>[2x]MQTRSSRMAGFGHAVPARCVDNAEIEASLGLEAGWIERRTGIRSRYWAEAGDTLSGLAERAGRMALEDAKINADDIALTLLATSTPDHLLPPSAPLLAHRLGLTRSGAIDLAGACSGFLYALTLADGFVRTYGRAVLVAAANILSRRINPAERASAVLFADAAGAVVLTPCPEVKRGVLSADLVADGSGYDLIQIAAGGSSQPFSAGMIAEDALMTMRDGREVFSRAVALMTNTSQRVLHEAELTAADISRFVPHQANARMSDAVCGNLGIEREKTVRTIGSFGNSSAATIPLSLSITNAERPLAGGETLLLTAAGAGMTGGAVVYRV

In contrast, a fabH-like gene, bioZ, seems to be domesticated into a unique bioBFDAZ operon in certain α-proteobacterial species. Genetic and biochemical characterization demonstrates that BioZ catalyzes the condensation of glutaryl-CoA (or ACP) with malonyl-ACP to give 5’-keto-pimeloyl ACP. This intermediate proceeds via type II fatty acid synthesis (FAS II) pathway, to initiate the formation of pimeloyl-ACP, a precursor of biotin synthesis. Thus, we proposed a working model that the α-proteobacterial BioZ enzyme behaves as an atypical member of β-ketoacyl-ACP synthase III to synthesize C7-fatty acyl moiety, bypassing the canonical ‘BioC-BioH’ earlier steps of pimelate generation.

Using X-ray crystallography, we crystallized and solved the structure of AtBioZ at a 1.99 Å resolution. The dimeric nature of the AtBioZ protein belongs to the space group of P 21 21 21 and contains two protomers in per asymmetric unit (ASU), of which the refinement statistics are listed in Table 1. The lid domain of AtBioZ contains four α-helices and two β-sheets, which is covering on the ‘α/β/α/β/α’ core domain. The core domain of AtBioZ features a triple decked sandwich that is formed by nine β-sheets and ten α-helices. In brief, the β-sheets of β1 and β4–β7 are sandwiched between the helices α3–α5 and α6, together with helices of α13–α14 to form the first layer, while the sheets of β8–β11 are sandwiched between the helices of α9–α12 and α6, together with the helix of α13–α14 to form the other layer of the “sandwich”. Interestingly, a putative catalytic triad (C115, H255, and N285) is centered in the core domain of AtBioZ. Structural alignment revealed that the root-mean-square deviation (rmsd) of Cα atoms of AtBioZ is 2.8, 2.7 , and 1.2 Å, in comparison with FabB, FabF, and FabH, respectively, while the rmsd between FabB and FabF is 1.4 Å. The diameter of substrate entrance of both AtBioZ and FabH is measured to be around 5 Å. The depth of the substrate-loading tunnel in AtBioZ is 20 Å, quite longer than the counterpart (15 Å) of FabB. Unlike that the FabB substrate-binding pocket whose entrance is close to the dimeric interface, the entrance of the AtBioZ substrate-binding pocket is relatively far away from the dimeric interface. Similarly, the surface around the entrance of BioZ pocket is enriched with positively-charged amino acids, namely Arg39, Arg153, Arg221, and Arg260. In particular, we localize that three residues (S84, R147, and S287) at the distant bottom of the tunnel might neutralize the charge of free C-carboxyl group of the primer glutaryl-CoA.> T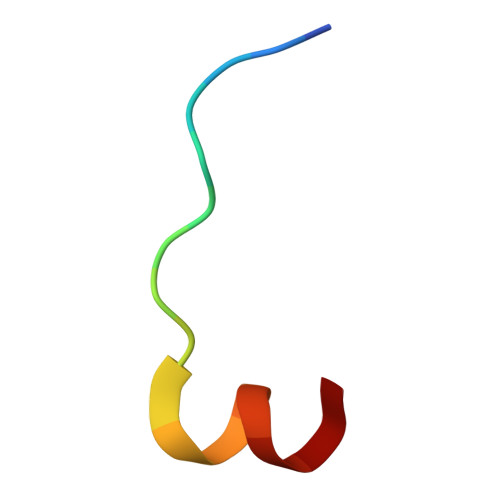GGKAPRKQLATKAARK2-PHENYLAMINO-4-METHYL-5-ACETYL THIAZOLE | C12 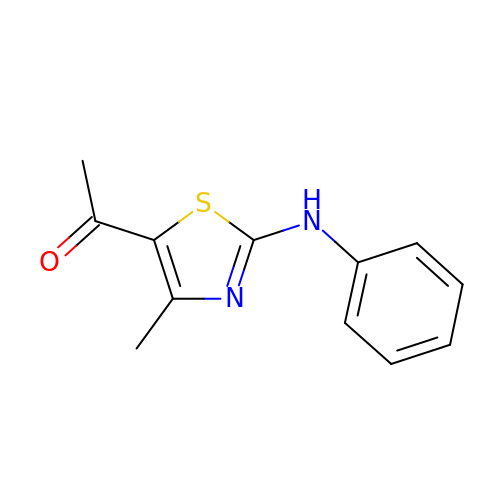H12 N2 O S | UIIUOFPGDKBCEZ-UHFFFAOYSA-N> TETTSFSITKFGPDQQNLIFQGDGYTTKERLTLTKAVRNTVGRALYSSPIHIWDSK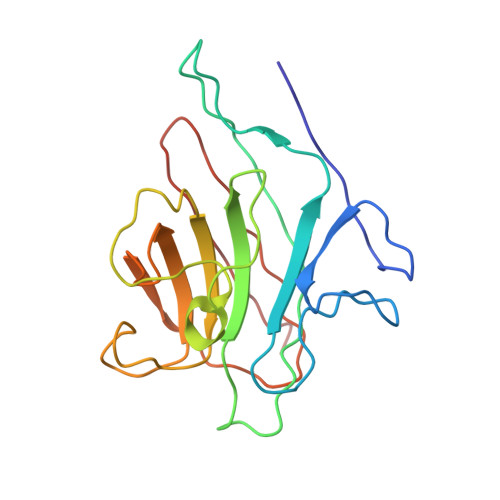TGNVANFVTSFTFVIDAPNSYNVADGFTFFIAPVDTKPQTGGGYLGVFNSKDYDKTSQTVAVEFDTFYNTAWDPSNGDRHIGIDVNSIKSINTKSWALQNGKEANVVIAFNAATNVLTVSLTYPN> MHHHHHHSSGRENLYFQGMSDTWSSIQAHKKQLDSLRERLQRRRKQDSGHLDLRNPEAALSPTFRSDSPVPTAPTSGGPKPSTASAVPELATDPELEKKLLHHLSDLALTLPTDAVSICLAISTPDAPATQDGVESLLQKFAAQELIEVKRGLLQDDAHPTLVTYADHSKLSAMM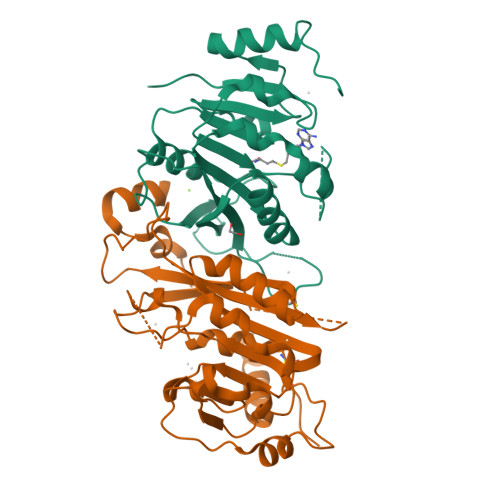GAVAEKKGPGEVAGTVTGQKRRAEQDSTTVAAFASSLVSGLNSSASEPAKEPAKKSRKHAASDVDLEIESLLNQQSTKEQQSKKVSQEILELLNTTTAKEQSIVEKFRSRGRAQVQEFCDYGTKEECMKASDADRPCRKLHFRRIINKHTDESLGDCSFLNTCFHMDTCKYVHYEIDACMDSEAPGSKDHTPSQELALTQSVGGDSSADRLFPPQWICCDIRYLDVSILGKFAVVMADPPWDIHMELPYGTLTDDEMRRLNIPVLQDDGFLFLWVTGRAMELGRECLNLWGYERVDEIIWVKTNQLQRIIRTGRTGHWLNHGKEHCLVGVKGNPQGFNQGLDCDVIVAEVRSTSHKPDEIYGMIERLSPGTRKIELFGRPHNVQPNWITLGNQLDGIHLLDPDVVARFKQKYPDGIISKPKNL;> MDSRLQEIRERQKLRRQLLAQQLGAESADSIGAVLNSKDEQREIAETRETCRASYDTSAPNAKRKYLDEGETDEDKMEEYKDELEMQQDEENLPYEEEIYKDSSTFLKGTQSLNPHNDYCQHFVDTGHRPQNFIRDVGLADRFEEYPKLRELIRLKDELIAKSNTPPMYLQADIEAFDIRELTPKFDVILLEPPLEEYYRETGITANEKCWTWDDIMKLEIDEIAAPRSFIFLWCGSGEGLDLGRVCLRKWGYRRCEDICWIKTNKNNPGKTKTLDPKAVFQRTKEHCLMGIKGTVKRSTDGDFIHANVDIDLIITEEPEIGNIEKPVEIFHIIEHFCLGRRRLHLFGRDSTIRPGWLTVGPTLTNSNYNAETYASYFSAPNSYLTGCTEEIERLRPKS> MSVVSQVILQADDQLRYPTSGELKGIQAFLTTGAQRIRIAETLAENEKKIVDQAQKQLFKKHPEYRAPGGNAYGQRQYNQCLRDYGWYLRLVTYGVLAGNKEPIETTGLIGVKEMYNSLNVPVPGMVDAVTVLKDAALGLLSAEDAN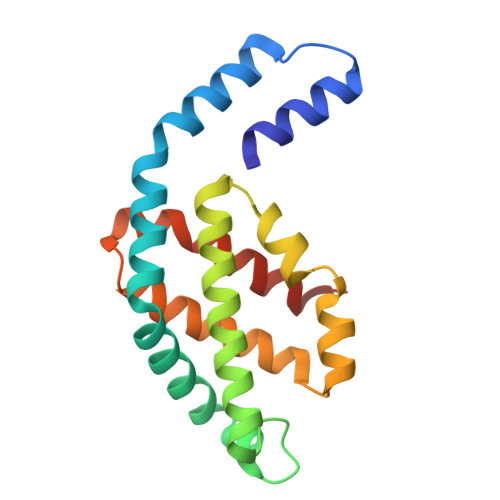ETAPYFDYIIQFMSHHHHHH>[6x]MGAAGDAAIGRESRELMSAADVGRTISRIAHQIIEKTALDDPVGPDAPRVVLLGIPTRGVTLANRLAGNITEYSGIHVGHGALDITLYRDDLMIKPPRPLASTSIPAGGIDDA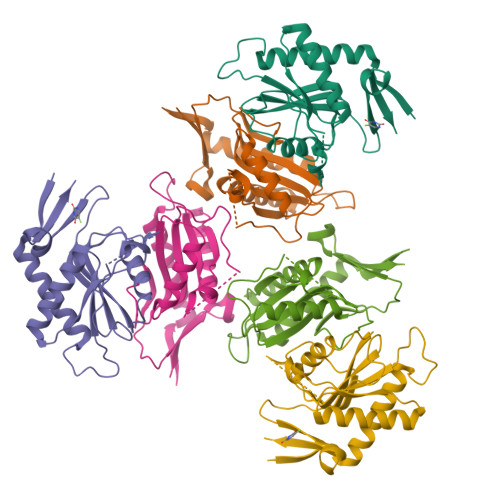LVILVDDVLYSGRSVRSALDALRDVGRPRAVQLAVLVDRGHRELPLRADYVGKNVPTSRSESVHVRLREHDGRDGVVISRHHHHHH>AKGSTNHRALTGVIFEPFEEVKKELDLVPTVPQASLARQKYVDESESAVNEQINVEYNVSYVYHAMFAYFDRDNVALRGLAKFFKESSEEEREHAEKLMEYQNKRGGKVKLQSIVMPLSDFDHADKGDALHAMELALSLEKLTNEKLLNLHSVATKNGDVQLADFVETEYLGEQVEAIKRIS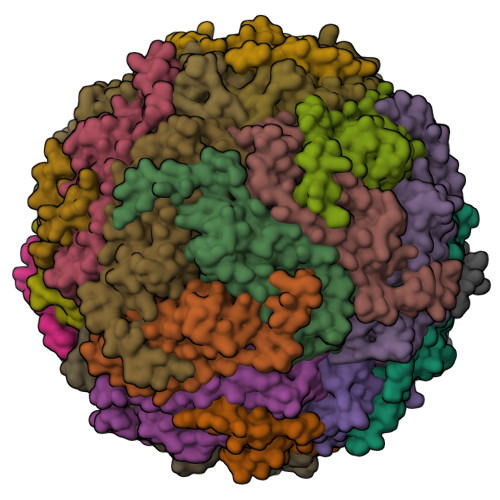EYVAQLRRVGKGHGVWHFDQMLLHEGGDAA[24x]2-(ACETYLOXY)BENZOIC ACID | C9 H8 O4 | 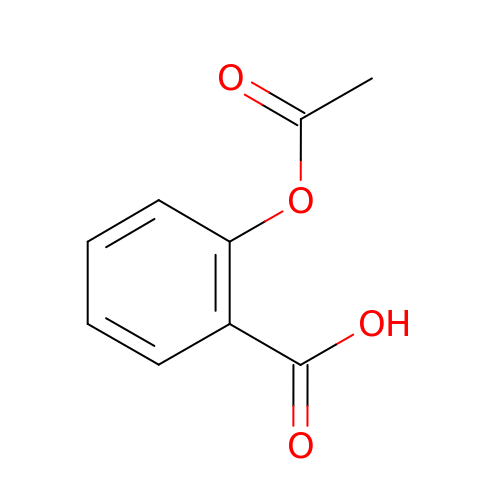BSYNRYMUTXBXSQ-UHFFFAOYSA-N>MTSLNDIVNKLSSSKIKTRSDALQNLRSYIIYSRNGNSLNQEDALIIEKAIKRAFELEWQISANHGKRQISKASQEQKLQDISYLLRTCVESYILLFREPHILALLDIILRHTFTANGSICEVVCLNFSKALRLLLSHSPHLHHLRFSDWQSLVSYCCQAIEKLSIAEETYVSDSEEEPISQKNYQEISIWKSHDVIRVKQEVVELIYVMRSLVQWYAAPINFVSEQLLKFFEFFFYAYTEETDAHLPALQCLFQLCAYAIPNCNDYSASVVLLVFKILINSDKWKRLDLRLQLIQCLAISYPLWSNSETWDPHRSIRSFNLDLLNSSFFSLKNFLNFFGKRSSLSLANFRFHTVEPKNNIAKLYDPRLHLFFSLRHNSFFESYFIYFFLAKLILLKKTVLSLASTEQANKKQKTCSQIEELLLQAELANISASSFSLQLMVIITAISDNLTNDDLLSIQKMSLNFTEKKNELQSWSFFILFNICYNKAYSSMLTTSCKKEILAAASRGLLNSVTSPVCYQILTYFNMYRPLCFASIFPFIKQQFILFNDYSPMLSYEAIDYWKSLYILLNENLFVGQSSFKSVFLKWLKWHLYHLFSKEGELPFFSFTDSSIIIFDLLMMIFYRPLSLSYITTEIRSPFERNLFHLKEAWSPVTLRFPYTTDEICKQSTEGCYPFNSNHTIDCDSLQNVIKMLESSIDEISSASYDKDELDKETPSFEAVMIFSQISFLCGFLNCFIQKKGIHNVTPNNLVIFKNLFPEVLSFVKSNHSYDPIINCISTNLQFTISDEPKHLRYEIGSDLIRSTHFRDSNPLKTLVLYIMDMASKNVFIKPQEFDHDEYFSQEEEDIYRPENLIRNHQILGLMEGSLEQIRNTDLFILQKYIDYFSSHPHDSLINILHLYPIETFCFGMSAIGAYFLDVARTSEPIFYKCLEILAQKILMNYDYERDEVYLMIFIKIFQKCVHSKLQFTDATLKLIVKITKFIEKVFIETKFSSLSGRQTFLKFIFQLSPTSHVYSKFDYQKLISLTLKDSDVCVIYNFVDDLVIFLKKCDKTLIEGFVLPILSIKIEKSLYKGFCYLYLTLKVFLSISSNRSALLYQLLKLANSYETSTIFEPLLRKLHIQSANIKQLFRIYRLEIFWSFVSKDLSNTTNDFLEFPYKPIYFSLSDFLKENSDEIILVLILTKNITLAKLITSRMSVDFSEKYTQLIPVITTYTHLSEVENKKYSLRFNSIDEALDVELLNRSKAFLFCLEMLKEVKELGSTFKSISSTSFKVYSQLTIFANRVSFNNSTAIPFFSTKSVLWYCNRLFQELEGFSSIPSVIDLVLRRLAIQLHFATDEELQVTISFRLCAFLCFSDPFITSNYLVMIVLRIARQLLSIPCTQSLGLGIARFHLKKFKPTDFDYFFQLAEFCMDFLGFCYNTIGTKMEAIQDFYTWFDGYVTALLNFEYEGYGFLRCQINFVRSVMTTKNEWIEVSNKLFERGHFLKRIAMNNYLCLYFWQVLDACPRNVLHSLSLEIWKCYKAYDITEFPDSLKLFFSDIMGWNFFKSPEIADLNHYIPKTDPRLCDTKTYEESKLIIWKLICQKACSLLFKYDILLDSFIEDCIRMFFENGNHQELRKFLNFPKDSIIYDSDFKTLVSEEGSFQWVKLQPTNFDSLSNWTKEETLKLLNMMGKSSTTHSLKLLSTYMVGFSTSIIQYIIHLILLEFDFNGNNKKQKEYVTQLILSGLLNKNTNSIRKTCMNILLYLRRQLGHHALNPFEANYWVPINYSVAASTAYDCHLYEQSLLFLTIHNTKTDELDITLLSDILSQLPCPDAYYGIKRETSFKNILLKAVHEKRSPLAISYLDAANMYRSNEDEGTKMMFSNTLNNAGFFSLNEFYIDSLKANDAIDECSNEVYASAWRMQKWDIPPLSLDNKTTKDCLVFEVLHAVHNYAIYGNYLHLEEYINKKLLLINPNEEPDSLLFYALAYDLKFLIRCNQSQFNCDILQLLKENKQMSSQLHECFQLLLEIRNVLLSLLQSHKQLDLSDDLASFRKYYILELLKISESFLIVDNLQNAFSVAMLSDALYRKFDLADENLKHDIDFLSSKILWQRDEKIDAIGMLSESLSKTNSSIFPSISYAYLGNWLYTTKSEKTELVSKNYFEKSLSHMSHLNAKEKAKIYCMFAQFCDNNYSSPDLTEDFKRMEKLYFEKKNDIQQLERSIVNASNMKEEKMLKNHHSREMSSFIIDEREYLRMSTFRSKMLTQSITHYLKCLSESDENDVLISRCCTMWLSNSHLDELNNSLQHYLQNLPCKKFIPVFYQLAARLMNENSKFQQSLTSICYNVGRNHPYHSLHVLFSLVSNVPEIENLDAGSRYRAVKKILDLLKVNQGLSNLVTKLLCSFENYVSLAEWNPRSKVDSTSFSRFPGYKWFLKDAANYGLPPITMNVKVNDTGDYSNIPTVSSFDDTIHFASGINAPKVITCLGSNGHTYKQLVKGGNDDLRQDAVMEQVFEQVNGFLRSYRKTSQRNLSMRTYKVIPLALKTGVIEWVQDTIPLGEYLDSAHKVYHPKEWSLSTCRKLIAEKQMEDLETRLKVYDLVCRHYRPVFRHFFLESYADPVQWFTTQTNYARSTAVASVLGHVLGLGDRHGQNILIDKTSGEVIHIDLGIAFEQGKKLPVPECVPFRLTRDVVDGMGITGVEGVFRRCMEFTLETLRREEDSLLSVLEVLRYDPLFSWLISPLRRMKKQKMQLENFNQPESGNITTDASRDPKIQRNNVSGESEAERAILKVRQKLSSTLSVEASVGELIRIAQDPSYLALMFCGWSAFQ[2x];> VSTQELYS

The ataxia–telangiectasia mutated (ATM), an apical kinase that orchestrates the multifaceted DNA damage response, is the master regulator of genome stability, and is a critical therapeutic target in cancer. ATM/Tel1 kinase functions as an obligate homodimer with a highly dynamic N-terminal helical solenoid domain responsible for ligand binding and a conserved C-terminal FAT/kinase/FATC domain6. However, the activation mechanism of ATM/Tel1 in response to DNA damage remains largely unknown.

After incubating the active wild-type ATM/Tel1 with the CHK2 substrate peptide (CHK263–74), and AMP-PNP in vitro, we froze the specimen and determined the cryo-EM reconstruction, which revealed that ATM/Tel1 adopts three distinct conformations. We focused on analyzing Structure 2 of the active state that binds to the substrate peptide, with a resolution of 3.6 Å. Unexpectedly, only one monomer in the active dimer binds to the substrate peptide. We designated the substrate-bound monomer as Mono1 and the other as Mono2. The hydroxyl group of the phospho-acceptor threonine (Thr68) in the peptide substrate is oriented towards the γ-phosphate of AMP-PNP, forming a hydrogen bond with His2632 in the catalytic loop. The glutamine (Gln69) sits in a hydrophobic pocket formed by the activation loop and the FATC domain, where it stacks against Phe2805 (FATC) and forms a pair of hydrogen bonds with the backbone of Val2662 (activation loop). However, the Lys2730 of the kα9b in the PIKK regulatory domain (PRD) of Mono2 occupies the Thr68-binding site, and Gln2731 occupies the Gln69-binding site, thereby competitively preventing substrate binding in the catalytic center. In the active form of Mono1, both kα9b and kα9c are disordered, enabling the substrate peptide to bind at the active site. In contrast, in the active state of Mono2, only kα9c is disordered, while kα9b remains in place, blocking access to the substrate-binding site. The Mono1 N-lobe packing against HEAT 34 R (residues 1583–1610) clamps the substrate peptide and defines a confined catalytic chamber, whereas the N-lobe docking at HEAT 32 R (residues 1470–1483) in Mono2 stabilizes a widened active center and facilitates substrate entry or product release.>AGNEFSSSGLGRAYSGEGAIADDAGNVSRNPALITMFDRPTFSAGAVYIDPDVNISGTSPSGRSLKADNIAPTAWVPNMHFVAPINDQFGWGASITSNYGLATEFNDTYAGGSVGGTTDLETMNLNLSGAYRLNNAWSFGLGFNAVYARAKIERFAGDLGQLVAGQIMQSPAGQTQQGQALAATANGIDSNTKTAHLNGNQWGFGWNAGILYELDKNNRYALTYRSEVKIDFKGNYSSDLNRAFNNYGLPIPTATGGATQSGYLTLNLPEMWEVSGYNRVDPQWAIHYSLAYTSWSQFQQLKATSTSGDTLFQKHEGFKDAYRIALGTTYYYDD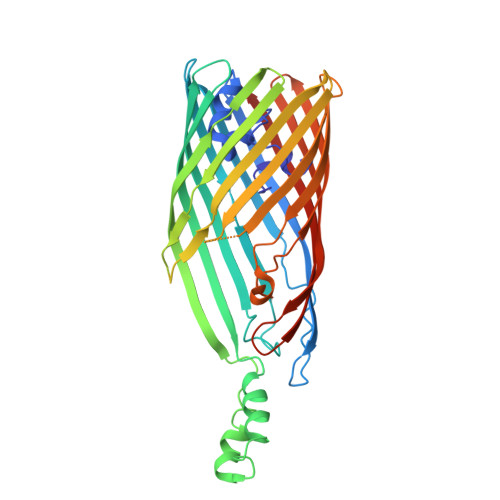NWTFRTGIAFDDSPVPAQNRSISIPDQDRFWLSAGTTYAFNKDASVDVGVSYMHGQSVKINEGPYQFESEGKAWLFGTNFNYAFHHHHHH[2x]> GSDKGKLSLQDVAELIRARACQRVVVMVGAGISTPSGIPDFRSPGSGLYSNLQQYDLPYPEAIFELP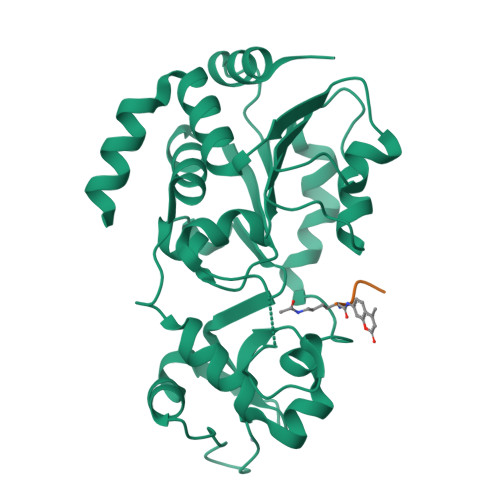FFFHNPKPFFTLAKELYPGNYKPNVTHYFLRLLHDKGLLLRLYTQNIDGLERVSGIPASKLVEAHGTFASATCTVCQRPFPGEDIRADVMADRVPRCPVCTGVVKPDIVFFGEPLPQRFLLHVVDFPMADLLLILGTSLEVEPFASLTEAVRSSVPRLLINRDLVGPLAWHPRSRDVAQLGDVVHGVESLVELLGWTEEMRDLVQRETGKLDGPDK>[3x]MAHNNENVSGISAYLLGLIIGDGGLYKLKYKGNRSEYRVVITQKSENLIKQHIAPLMQFLIDELNVKSKIQIVKGDTRYELRVSSKKLYYYFANMLERIRLFNMREQ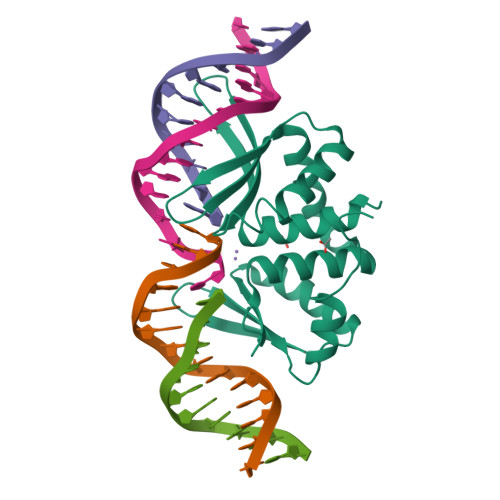IAFIKGLYVAEGDKTLKRLRIWNKNKALLEIVSRWLNNLGVRNTIHLDDHRHGVYVLNISLRDRIKFVHTILSSHLNPLPPEAAALEHHHHHH>[4x]MIEKQMDRVVKEMR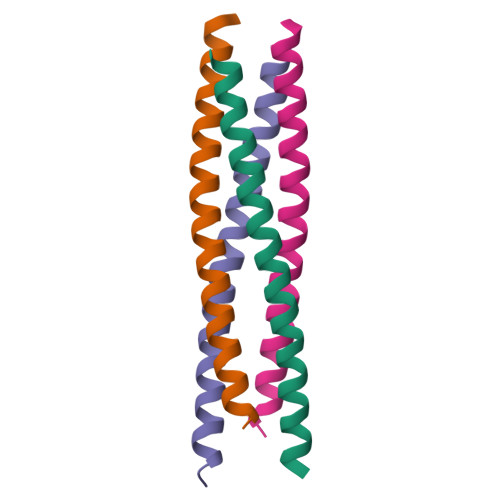RQLEMIDKLTTRGIEQVELLKRIHDKLMIRAVD>[2x]APRKFFVGGNWKMNGDKKSLGELIHTLNGAKLSADTEVVCGAPSIYLDFARQKLDAKIGVAAQ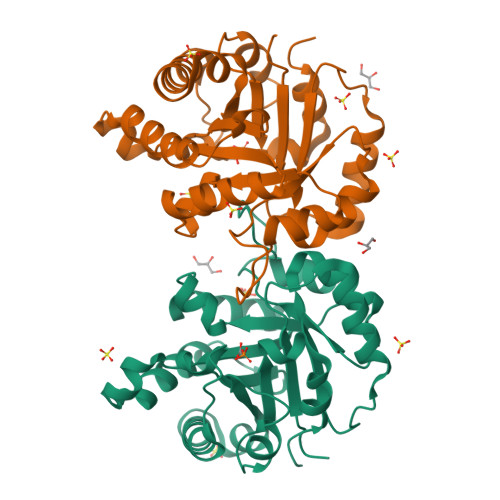NCYKVPKGAFTGEISPAMIKDIGAAWVILGHSERRHVFGESDELIGQKVAHALAEGLGVIACIGEKLDEREAGITEKVVFEQTKAIADNVKDWSKVVLAYEPVWAIGTGNPNTPQQAQEVHEKLRGWLKSHVSDAVAQSTRIIYGGSVTGGNCKELASQHDVDGFLVGGASLKPEFVDIINAKH>[2x]MKFTVEREHLLKPLQQVSGPLGGRPTLPILGNLLLQVADGTLSLTGTDLEMEMVARVALVQPHEPGATTVPARKFFDICRGLPEGAEIAVQLEGERMLVRSGRSRFSLSTLPAADFPNLDDWQSEVEFTLPQATMKRLIEATQFSMAHQDVRYYLNGMLFETEGEELRTVATDGHRLAVCSMPIGQSLPSHSVIVPRKGVIELMRMLDGGDNPLRVQIGSNNIRAHVGDFIFTSKLVDGRFPDYRRVL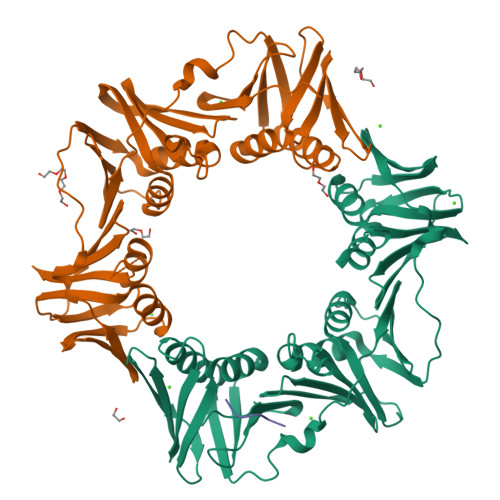PKNPDKHLEAGCDLLKQAFARAAILSNEKFRGVRLYVSENQLKITANNPEQEEAEEILDVTYSGAEMEIGFNVSYVLDVLNALKCENVRMMLTDSVSSVQIEDAASQSAAYVVMPMRL;> XQLALF> MSGSLKSLDKKIAKRRQVYKPVLDNPFTNEAHMWPRVHDQPLIWQLLQSSIINKLIHIQSKENYPWELYTDFNEIVQYLSGAHGNSDPVCLFVCNKDPDVPLVLLQQIPLL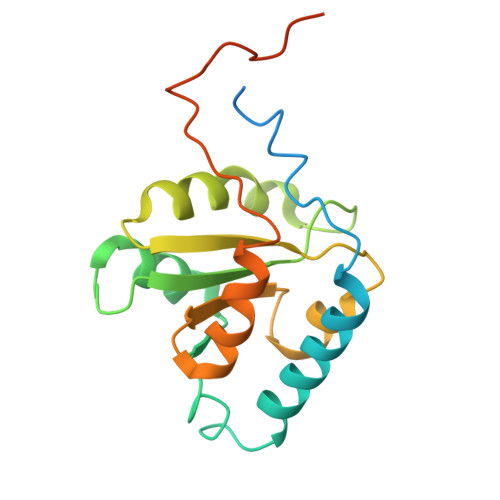CYMAPMTVKLVQLPKSAMDTFKSVSKYGMLLLRCDDRVDKKFVSQIQKNVDLLQFPWLNAIKYRPTSVKLLKTTVPIVSKKRQK>[2x]SNAMNIRTELQNSQLCEGITEAQLTELMNKITVKEKHYK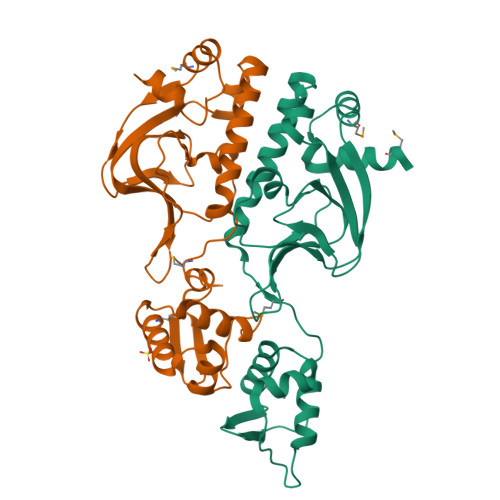NNEILFYTDEVTKVYILVKGNAAIAKNTSSGKRILGKNVTEPGELAGEIYYFSHRNPFWDYAIVLEPTTVLEISGIDQGTLQTLDLALQNQLLVNLLKSVTRKFEYIGEKVRMVSEDSVRAKISNYLFGIQDDDGSIELTETREEIADYLDITRPSLSRELGRMQKENIIRIEGSSVIILDAIIFDTFIE>MAEAGLRGWLLWALLLRLAQSEPYTTIHQPGYCAFYDECGKNPELSGSLMTLSNVSCLSNTPARKITGDHLILLQKICPRLYTGPNTQACCSAKQLVSLEASLSITKALLTRCPACSDNFVNLHCHNTCSPNQSLFINVTRVAQLGAGQLPAVVAYEAFYQHSFAEQSYDSCSRVRVPAAATLAVGTMCGVYGSALCNAQRWLNFQGDTGNGLAPLDITFHLLEPGQAVGSGIQPLNEGVARCNESQGDDVATCSCQDCAASCPAIARPQALDSTFYLGQMPGSLVLIIILCSVFAVVTILLVGFRVAPARDKSKMVDPKKGTSLSDKLSFSTHTLLGQFFQGWGTWVASWPLTILVLSVIPVVALAAGLVFTELTTDPVELWSAPNSQARSEKAFHDQHFGPFFRTNQVILTAPNRSSYRYDSLLLGPKNFSGILDLDLLLELLELQERLRHLQVWSPEAQRNISLQDICYAPLNPDNTSLYDCCINSLLQYFQNNRTLLLLTANQTLMGQTSQVDWKDHFLYCANAPLTFKDGTALALSCMADYGAPVFPFLAIGGYKGKDYSEAEALIMTFSLNNYPAGDPRLAQAKLWEEAFLEEMRAFQRRMAGMFQVTFMAERSLEDEINRTTAEDLPIFATSYIVIFLYISLALGSYSSWSRVMVDSKATLGLGGVAVVLGAVMAAMGFFSYLGIRSSLVILQVVPFLVLSVGADNIFIFVLEYQRLPRRPGEPREVHIGRALGRVAPSMLLCSLSEAICFFLGALTPMPAVRTFALTSGLAVILDFLLQMSAFVALLSLDSKRQEASRLDVCCCVKPQELPPPGQGEGLLLGFFQKAYAPFLLHWITRGVVLLLFLALFGVSLYSMCHISVGLDQELALPKDSYLLDYFLFLNRYFEVGAPVYFVTTLGYNFSSEAGMNAICSSAGCNNFSFTQKIQYATEFPEQSYLAIPASSWVDDFIDWLTPSSCCRLYISGPNKDKFCPSTVNSLNCLKNCMSITMGSVRPSVEQFHKYLPWFLNDRPNIKCPKGGLAAYSTSVNLTSDGQVLTSRFMAYHKPLKNSQDYTEALRAARELAANITADLRKVPGTDPAFEVFPYTITNVFYEQYLTILPEGLFMLSLCLVPTFAVSCLLLGLDLRSGLLNLLSIVMILVDTVGFMALWGISYNAVSLINLVSAVGMSVEFVSHITRSFAISTKPTWLERAKEATISMGSAVFAGVAMTNLPGILVLGLAKAQLIQIFFFRLNLLITLLGLLHGLVFLPVILSYVGPDVNPALALEQKRAEEAVAAVMVASCPNHPS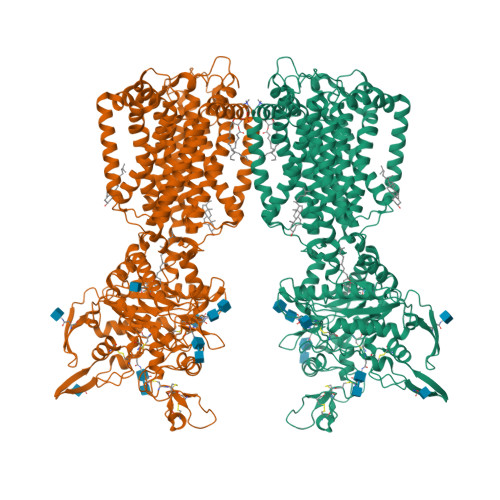RVSTADNIYVNHSFEGSIKGAGAISNFLPNNGRQF[2x]(2S)-2-[[(2S)-2-[2-[(2-azanyl-4-oxidanylidene-3H-pteridin-7-yl)carbonylamino]ethanoylamino]-3-phenyl-propanoyl]amino]-6-(phenylmethoxycarbonylamino)hexanoic acid | C32 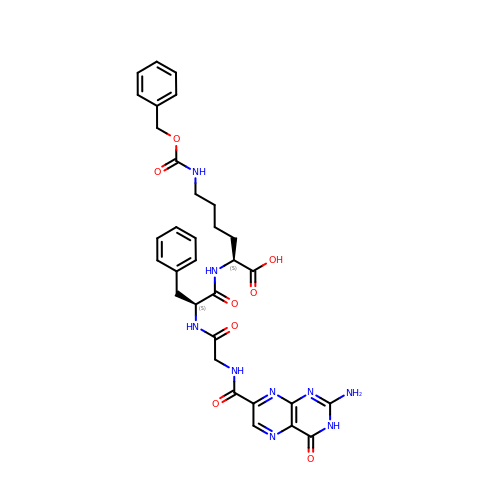H35 N9 O8 | FVYSJCKPWXGJBU-VXKWHMMOSA-N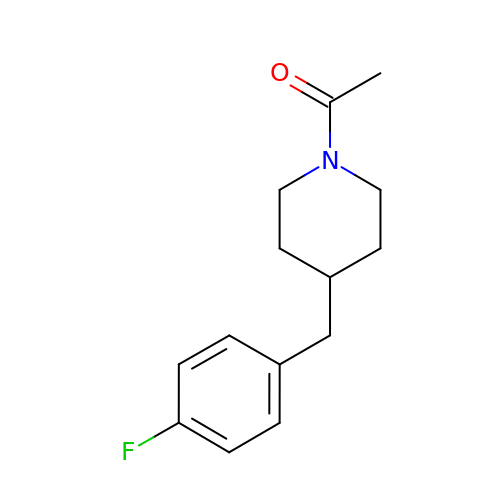1-[4-[(4-fluorophenyl)methyl]piperidin-1-yl]ethanone | C14 H18 F N O | OOMYIKQRRZLESA-UHFFFAOYSA-N>GEGMWVPQQLPEIAGPLKKAGLKLSPQQISDLTGDPMGAVVALGGCTASFVSPNGLVVTNHHCAYGAIQLNSTAENNLIKNGFNAPTTADEVSAGPNARVFVLDEITDVTKDAKAAIAAAGDDALARTKALEAFEKKLIADCEAEAGFRCRLYSFSGGNTYRLFKNLEIKDVRLAYAPPGSVGKFGGDIDNWMWPRHTGDFAFYRAYVGKDGKPAAFSKDNVPYQPKHWLKFADQPLGAGDFVMVAGYPGSTNRYALAAEFDNTAQWTYPTIARHYKNQIAMVEAAGKQNADIQVKYAATMAGWNNTSKNYDGQLEGFKRIDAAGQKLREEAAVLGWLKGQGAKGQPALDAHAKLLDLLEQSKATRDRDLTLALFNNTAMLGSATQLYRLSIEREKPNAERESGYQERDLPAIEGGLKQLERRYVAAMDRQLQEYWLNEYIKLPADQRVAAVDAWLGGNDAAAVKRALDRLAGTKLGSTEERLKWFAADRKAFEASNDPAIQYAVAVMPTLLK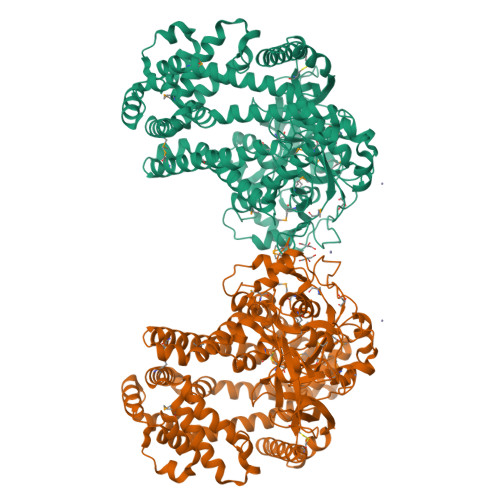LEQERKTRAGENLAARPVYLQALADYKKSQGEFVYPDANLSLRITFGNVMGYAPKDGMEYTPFTTLEGVVAKETGQDPFDSPKALLDAVAAKRYGGLEDKRIGSVPVNYLSDLDITGGNAGSPVLDAHGKLVGLAFDGNWESVSSNWVFDPKMTRMIAVDGRYLRWIMQEVYPAPQLLKEMNVGK[2x]The E301R protein (pE301R) from ASFV was previously predicted as a proliferating cell nuclear antigen (PCNA)-like protein through clamping DNA polymerase to the DNA duplex, but its exact structure and functions remain uncharacterized. Here, the crystal structure of pE301R revealed that it is composed of structurally similar head and tail domains and shares significant structural similarities to the DNA polymerase processivity factors, including sliding clamp and eukaryotic PCNA. We demonstrate that the protein displays a ring-shaped homotetramer and functions as a viral analog of the sliding clamp. Taken together, we revealed that pE301R functions as a sliding clamp in ASFV genomic replication and can be used as a potential antiviral target.

To gain insights into pE301R functions, we determined its crystal structure using the single-wavelength anomalous dispersion method with the selenomethionine (Se-Met)-labeled proteins. The residues 15–162 and 165–301 could be observed in the density map that was built in the final model. The structure contains four α-helices (α1–4) and 18 β-sheets (β1–18), which could be divided into two globular similar subdomains (named as the head domain: α1–2 and β1–9 and the tail domain: α3–4/β10–18). The head and tail domains are connected by an inter-domain connecting loop (IDCL) mixed with a short helix (η1). Inspection of the crystal packing of the pE301R structure revealed that it could form a homotetramer ring with the neighboring molecules in a head-to-tail manner, around a crystallographic fourfold axis with pseudo-eightfold symmetry. The assembly of the tetramer produces a central channel of approximately 52 Å in diameter. The homotetramer is mediated by the interactions mainly between β9 in one subunit and β13 in another one via multiple hydrogen bonds/salt bridges as well as hydrophobic contacts. For example, the side chain of K148 of one subunit forms two salt bridges with the side chains of E230 of neighboring subunit, while Y152 of one subunit generates hydrophobic aromatic stackings with Y228 and F223 of neighboring subunit, to stabilize the contacts between the two protomers. The inner surface of the ring is composed of the 16 helices (α1–4 from each of the four protomers) that are oriented to form a central hole that can encircle double-stranded DNA and allow its sliding like PCNA. Inspection of the charge distribution of the tetrameric ring revealed that its inner cavity has a positively charged surface distributed with many basic residues (lysine and arginine).

> MSEDIRRGPGRPPKKRVVPNFERKGILEKPVRPQSRLEFSYDNPLIFKNLFIYFKNLKSKNILVRCTPTEITFFSRDQSQASFVIATIDGKNVNHYYASDVFWLGINRELVEKMFNSIDRSFLKITIVHRYDKPETLFFIFTDFDIDKECTYQITVSEPELDMDLIEMEKSISEERLKNYPLRWEFTSKQLKKTFSDLSNYTELVTIEKLGGDTPLHLYFQKFNSISYHEMYKSSNKINLTSTIPKSQVFQINVKIAHIKSLASAMVTDKIRILCEENGNLIFQSEMDALMLNTITLNNTI>[2x]MGSDKIHHHHHHMILKRAYDVTPQKISTDKVRGVRKRVLIGLKDAPNFVMRLFTVEPGGLIDRHSHPWEHEIFVLKGKLTVLKEQGEETVEEGFYIFVEPNEIHGFRNDTDSEVEFL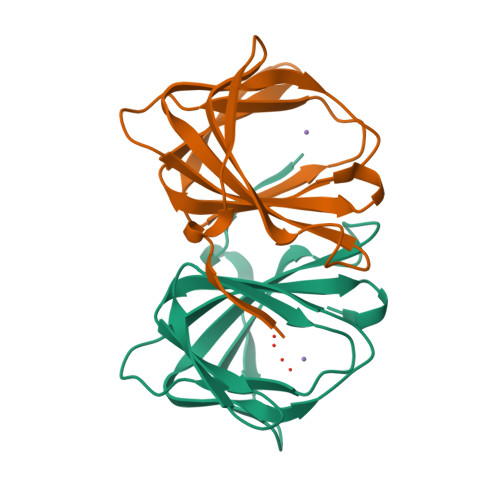CLIPKEGGE> MTTTERPDLAWLDEVTMTQLERNPYEVYERLRAEAPLAFVPVLGSYVASTAEVCREVATSPDFEAVITPAGGRTFGHPAIIGVNGDIHADLRSMVEPALQPAEVDRWIDDLVRPIARRYLERFENDGHAELVAQYCEPVSVRSLGDLLGLQEVDSDKLREWFAKLNRSATNAAVDENGEFANPEGFAEGDQAKAEIRAVVDPLIDKWIEHPDDSAISHWLHDGMPPGQTRDREYIYPTIYVYLLGAMQEPGHGMASTLVGLFSRPEQLEEVVDDPTLIPRAIAEGLRWTSPIWSATARISTKPVTIAGVDLPAGTPVMLSYGSANHDTGKYEAPSQYDLHRPPLPHLAFGAGNHACAGIYFANHVMRIALEELFEAIPNLERDTREGVEFWGWGFRG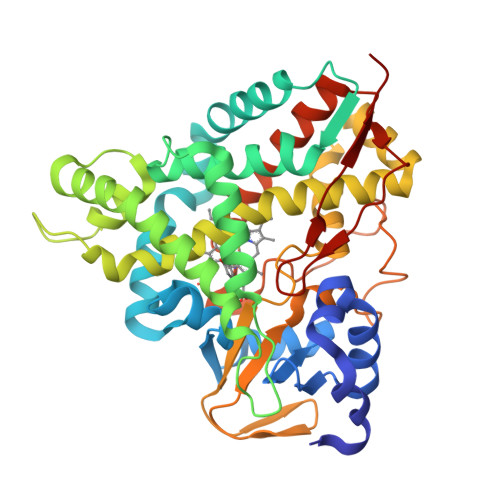PTSLHVTWEV>[2x]MKYKAVLVDFGNTLVGFKPVFYEKVYQVLKDNGYDLDLRKVFRAYAKAMGMINYPDED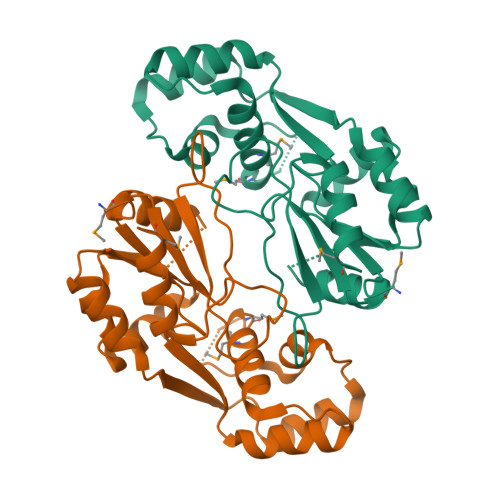GLEHVDPKDFLYILGIYPSERLVKELKEADIRDGEAFLYDDTLEFLEGLKSNGYKLALVSNASPRVKTLLEKFDLKKYFDALALSYEIKAVKPNPKIFGFALAKVGYPAVHVGDIYELDYIGAKRSYVDPILLDRYDFYPDVRDRVKNLREALQKIEEMNKE Wnt signalosome assembly relies on reversible head-to-tail polymerization by the N-terminal DIX domain of Dishevelled (Schwarz-Romond et al., 2007), which enables this hub to transduce Wnt signals to cytoplasmic effectors. In addition to DIX, Dishevelled has a PDZ domain (Post-synaptic density protein-95, Disc large tumor suppressor, Zonula occludens-1) and a DEP domain (Dishevelled, Egl-10, and Pleckstrin), separated by long flexible linkers peppered with phosphorylation sites, and also a binding motif for the AP2 clathrin adaptor (Yu et al., 2010). Here, we use structural analysis, as well as biophysical and cell-based assays, to show that the DEP domain of Dishevelled undergoes a conformational switch, from monomeric to swapped dimer, to trigger DIX-dependent polymerization and signaling to β-catenin. This occurs in two steps: binding of monomeric DEP to Frizzled followed by DEP domain swapping triggered by its high local concentration upon Wnt-induced recruitment into clathrin-coated pits.

Purifying lipoyl-tagged DEP (Lip-DEP416–511) by size exclusion chromatography (SEC), we observed two main peaks, corresponding to monomers and dimers (discussed later), in addition to a higher mass species. Thus, we crystallized the monomeric and dimeric fractions and determined three structures at 1.84–2.06 Å resolution. Remarkably, each structure exhibits a swapped dimer, regardless of the crystal form: namely, molecule A (turquoise) donates H1 to the H2–H3 core of molecule B (light turquoise) by extending loop 1, and vice versa. Thus, two DEP cores are connected by an extended β sheet, composed of two antiparallel β strands (each made up by a β1β2 tandem) that interact with each other through backbone atoms of residues 442–447. This dimer-specific interface is based on six new hydrogen bonds, which may bias the equilibrium toward the domain-swapped configuration. Interestingly, the solvent-exposed “underside” of the connecting β sheet presents a hydrophobic patch, made up of a triad of hydrophobic amino acids (M443, L445, and I447) located at the DEP finger tip of the monomer. In each crystal, two DEP dimers associate with each other through this hydrophobic patch, thus linking four DEP cores into a cross-shaped tetramer. The hydrodynamic radius of the dimer determined during SEC-MALS confirmed that its shape in solution is larger than a typical globular fold of 44 kDa mass, consistent with the extended configuration of the swapped dimer seen in the crystal. The dimerization defect resulting from mutating E499 and D460 can be rationalized by a striking salt-bridge network between their negatively charged side chains and the guanidinium group of a key arginine (R472). Notably, E499 is located on the loop between β3 and β4, and its salt bridge with R472 appears to be mainly responsible for tucking this loop under the DEP core.

>SSGLSVHTDMASVTKAMAAPESGLEVRDRMWLKITIPNAFLGSDVVDWLYHHVEGFPERREARKYASGLLKAGLIRHTVNKITFSEQCYYVFGDLSG[4x]To gain understanding into the function of the cytadherence machinery of mycoplasmas, in this study we have determined the crystal structure of P110, a major adhesin of M. genitalium and an immunodominant protein of this emergent sexually transmitted pathogen. P140 and P110, which have been shown to be reciprocally stabilized, interact to form a transmembrane complex, called “Nap”, that accumulates at a polar structure known as the terminal organelle. The structure of the extracellular region of P110 is composed by two domains, the N- and C-domains, very different in size, with an overall shape and domain organization that can be sketched as the body and the stalk of capital letter P. Within the N-domain of P110, long connections between some blades and also between some β-strands create a structure, referred as “the crown”, containing a binding site for sialic acid oligosaccharides, as conclusively shown by the structures of the complexes of P110 with both 3′- and 6′-sialyllactose oligosaccharides.

Co-crystallization of erP110 with either 3′-sialyllactose (3SL: where the neuraminic acid forms an α2–3 linkage to a lactose monosaccharide) or 6′-sialyllactose (6SL: with an α2–6 linkage) resulted in complexes of both oligosaccharides with erP110, as determined at 2.2 and 2.5 Å resolution, respectively (Experimental procedures section). The oligosaccharides binding site, the same for both complexes, is located in an indent of erP110 in the upper part of the crown. In both complexes only the neuraminic acid moiety presents direct interactions with two short stretches of the protein: Pro197–Ser198–Pro199–Asn200 and Ser456–Phe457–Ser458. The carboxylate group from the neuraminic acid forms two hydrogen bonds with Ser458, one with the backbone amino group and the second with the side chain oxygen. Finally, the methyl group of the neuraminic acid is placed into a hydrophobic pocket close to the Phe457 side chain. In the refined structures, oligosaccharides present different occupancies (∼100% for 6SL and ∼60–70% for 3SL), which suggest different binding affinities in spite of the fact that neuraminic acid is making about the same interactions in both complexes. The lactose moiety of 6SL is also well defined in the 6SL complex, while density is progressively weaker for 3SL suggesting that, beyond the neuraminic acid, the conformation of this oligosaccharide can fluctuate. The third monosaccharide approaches the protein in 6SL, while it is projected towards the solvent in 3SL. Affinity between erP110 and the sialic acid compounds was experimentally characterized by Surface Plasmon Resonance using biotinylated 3SL and 6SL immobilized on a streptavidin chip.

> ALANTFLVKEDSKNVTAYTPFATPITDSKSDLVSLAQLDSSYQIADQTIHNTNLFVLFKSRDVKVKYESSGSNNISFDSTSQGEKPSYVVEFTNSTNIGIKWTMVKKYQLDVPNVSSDMNQVLKNLILEQPLTKYTLNSSLAKEKGKTQREVHLGSGQANQWTSQRNQHDLNNNPSPNASTGFKLTTGNAYRKLSESWPIYEPIDGTKQGKGKDSSGWSSTEENEAKNDAPSVSGGGSSSGTFNKYLNTKQALESIGILFDDQTPRNVITQLYYASTSKLAVTNNHIVVMGNSFLPSMWYWVVERSAQENASNKPTWFANTNLDWGEDKQKQFVENQLGYKETTSTNSHNFHSKSFTQPAYLISGIDSVNDQIIFSGFKAGSVGYDSSSSSSSSSSSTKDQALAWSTTTSLDSKTGYKDLVTNDTGLNGPINGSFSIQDTFSFVVPYSGNHTNNGTTGPIKTAYPVKKDQKSTVKINSLINATPLNSYGDEGIGVFDALGLNYNFKSNQERLPSRTDQIFVYGIVSPNELRSAKSSADSTGSDTKVNWSNTQSRYLPVPYNYSEGIIDADGFKRPENRGASVTTFSGLKSIAPDGFANSIANFSVGLKAGIDPNPVMSGKKANYGAVVLTRGGVVRLNFNPGNDSLLSTTDNNIAPISFSFTPFTAAESAVDLTTFKEVTYNQESGLWSYIFDSSLKPSHDGKQTPVTDNMGFSVITVSRTGIELNQDQATTTLDVAPSALAVQSGIQSTTQTLTGVLPLSEEFSAVIAKDSDQNKIDIYKNNNGLFEIDTQLSNSVATNNGGLAPSYTENRVDAWGKVEFADNSVLQARNLVDKTVDEIINTPEILNSFFRFTPAFEDQKATLVATKQSDTSLSVSPRIQFLDGNFYDLNSTIAGVPLNIGFPSRVFAGFAALPA Norovirus (formerly Norwalk-like virus, NV) is a genus of the Caliciviridae family that is a major causative agent of non-bacterial acute gastroenteritis in humans. Among these, nonstructural protein 7 [RNA-dependent RNA polymerase (RdRp) domain] plays a key role in genome replication, as well as in the synthesis and amplification of additional subgenomic RNA. Notably, since RdRp is not present in mammalian cells, it appears as a suitable target for inhibition in the context of antiviral prophylaxis. Inspection of the crystal structures showed that 6 binds to a site located in the polymerase thumb domain, more specifically in a cleft along the exit path for the newly synthesized RNA.

6 diffraction data were collected at 100 K at the ESRF beam line ID29 (Grenoble, France); the crystal structure was solved by MR (2.3 Å resolution) and refined to final crystallographic R-factor/R-free values of 18.5/24.8%. Six mNV-RdRp molecules are hosted in the crystal asymmetric unit. Inspection of the refined model shows that the naphthalene disulphonate head of the inhibitor binds to the same RdRp location identified for hNV-RdRp. In the murine protein compound 6 could be fully modeled in all the subunits of the crystal asymmetric unit. The observed roto-translation of the ligand is related to the loss of the interaction with Gln439 and with His433, both pointing toward the solvent in mNV RdRp. Such shift of the ligand molecule promotes the stacking interaction of the toluene group of 6 with Arg392 guanidine moiety (H-bonded to 6 carbonyl, and in electrostatic interaction with 2 sulphonates), which allows the stabilization of the entire inhibitor. On the contrary in the mNV-RdRp/6 structure, the inhibitor could be completely modeled thanks to the different disposition of the naphthalene head due to the loss of the interaction with His433. On the contrary, the higher inhibitory potency of 6 against mNV-RdRp correlates with a fully defined binding mode and interactions of the inhibitor to the RdRp active site.

>[6x]MLPRPSGTYAGLPIADYGDAPPLSTKTMFWRTSPEKLPPGAWEPAYLGSKDERVDGPSLQQVMRDQLKPYSEPRGLLPPQEILDAVCDAIENRLENTLEPQKPWTFKKACESLDKNTSSGYPYHKQKSKDWTGSAFIGDLGDQATHANNMYEMGKSMRPIYTAALKDELVKPDKIYGKIKKRLLWGSDLGTMIRAARAFGPFCDALKETCIFNPIRVGMSMNEDGPFIFARHANFRYHMDADYTRWDSTQQRAILKRAGDIMVRLSPEPDLARVVMDDLLAPSLLDVGDYKIVVEEGLPSGCPCTTQLNSLAHWILTLCAMVEVTRVDPDIVMQESEFSFYGDDEVVSTNLELDMVKYTMALRRYGLLPTRADKEEGPLERRQTLQGISFLRRAIVGDQFGWYGRLDRASIDRQLLWTKGPNHQNPFETLPGHAQRPSQLMALLGEAAMHGEKYYRTVASRVSKEAAQSGIEMVVPRHRSVLRWVRFGTMDAETPQERSAVFVNEDELEHHHHHH> GPHMRVRLKAHYGGDILITSVDPTTTFQDLCEEVRDMCGLHQQHPLTLKWVDSEGDPCTVSSQMELEEAFRLACQGRDEVLI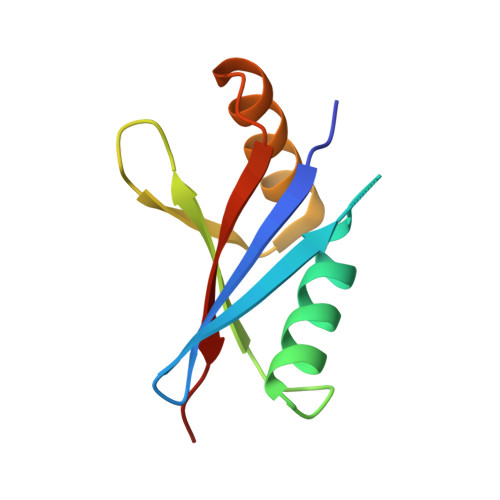IHVFPSIPE tetradecanethial | C14 H28 S | 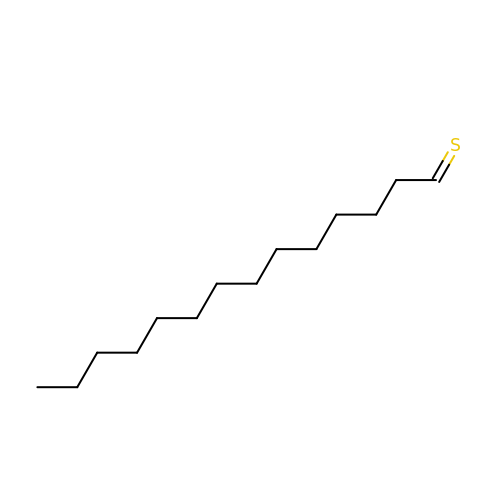JIHBDFISBDNMMA-UHFFFAOYSA-N Charcot–Marie–Tooth disease (CMT) is the most common inherited peripheral polyneuropathy in humans, and its different subtypes are linked to mutations in dozens of different genes. Mutations in ganglioside‐induced differentiation‐associated protein 1 (GDAP1) cause two types of CMT, demyelinating CMT4A and axonal CMT2K. The GDAP1‐linked CMT genotypes are mainly missense point mutations. Structural analysis of GDAP1 indicates that CMT may arise from disruption of specific intra‐ and intermolecular interaction networks, leading to alterations in GDAP1 structure and stability, and, eventually, insufficient motor and sensory neuron function.

Using GDAP1 variant crystal structures, we identify a side‐chain interaction network between helices ⍺3, ⍺6, and ⍺7, which is affected by CMT mutations, as well as a hinge in the long helix ⍺6, which is linked to structural flexibility.

>[4x]EVKLILYHWTHSFSSQKVRLVIAEKALKCEEHDVSLPLSEHNEPWFMRLNSTGEVPVLIHGENIICEATQIIDYLEQTFLDERTPRLMPDKESMYYPRVQHYRELLDSLPMDAYTHGCILHPELTVDSMIPAYATTRIRSQIGNTESELKKLAEENPDLQEAYIAKQKRLKSKLLDHDNVKYLKKILDELEKVLDQVETELQRRNEETPEEGQQPWLCGESFTLADVSLAVTLHRLKFLGFARRNWGNGKRPNLETYYERVLKRKTFNKVLG> SQETF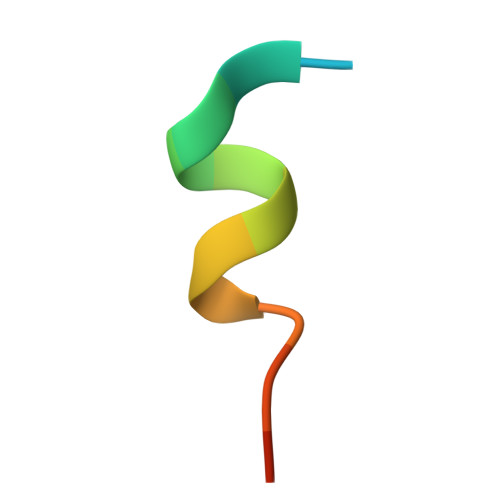SDLWKLLPEN> APAVADKADNAFMMICTALVLFMTIPGIALFYGGLIRGKNVLSMLTQVTVTFALVCILWVVYGYSLAFGEGNNFFGNINWLMLKNIELTAVMGSIYQYIHVAFQGSFACITVGLIVGALAERIRFSAVLIFVVVWLTLSYIPIAHMVWGGGLLASHGALDFAGGTVVEINAAIAGLVGAYLIGKRVGFGKEAFKPHNLPMVFTGTAILYIGWFGFNAGSAGTANEIAALAFVNTVVATAAAILGWIFGEWALRG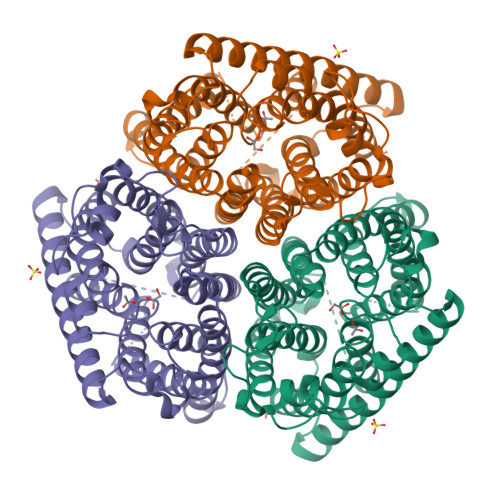KPSLLGACSGAIAGLVGVTPACGYIGVGGALIIGVVAGLAGLWGVTMLKRLLRVDDPCDVFGVHGVCGIVGCIMTGIFAASSLGGVGFAEGVTMGHQLLVQLESIAITIVWSGVVAFIGYKLADLTVGLRVPEEQEREGLDVNSHGENAYNADQAQQPAQADLEHHHHHH> GTHMVGMSGIGLWLKSLRLHKYIELFKNMTYEEMLLITEDFLQSVGVTKGASHKL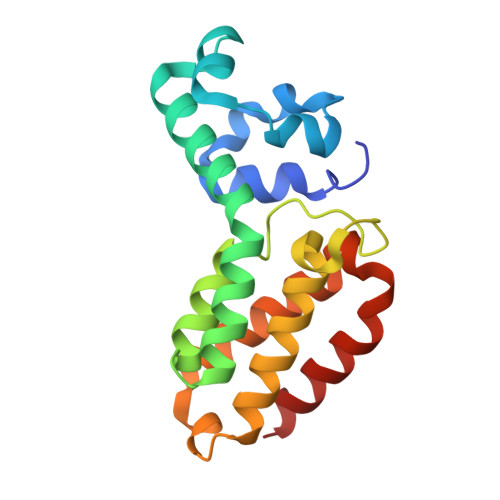ALCIDKLKERANILNRVEQELLSGQMELSTAVEELTNIVLTPMKPLESPGPPEENIGLRFLKVIDIVTNTLQQDPYAVQDDETLGVLMWILDRSIHNEAFMNHASQLKDLKFKLSKMK>[2x]ASAWPEEKNYHQPAILNSSALRQIAEGTS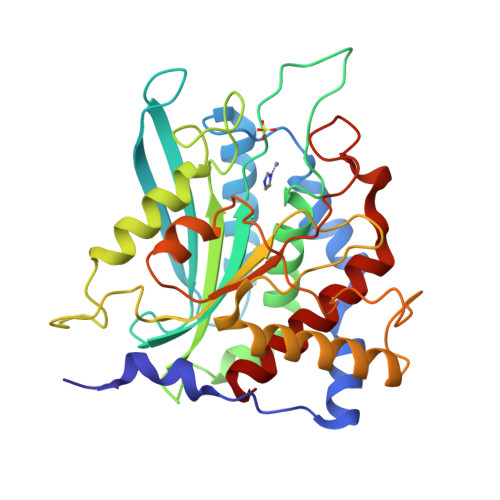ISEMWQNDLQPLLIERYPGSPGSYAARQHIMQRIQRLQADWVLEIDTFLSQTPYGYRSFSNIISTLNPTAKRHLVLACHYDSKYFSHWNNRVFVGATDSAVPCAMMLELARALDKKLLSLKTVSDSKPDLSLQLIFFDGLEAFLHWSPQDSLYGSRHLAAKMASTPHPPGARGTSQLHGMDLLVLLDLIGAPNPTFPNFFPNSARWFERLQAIEHELHELGLLKDHSLEGRYFQNYSYGGVIQDDHIPFLRRGVPVLHLIPSPFPEVWHTMDDNEENLDESTIDNLNKILQVFVLEYLHL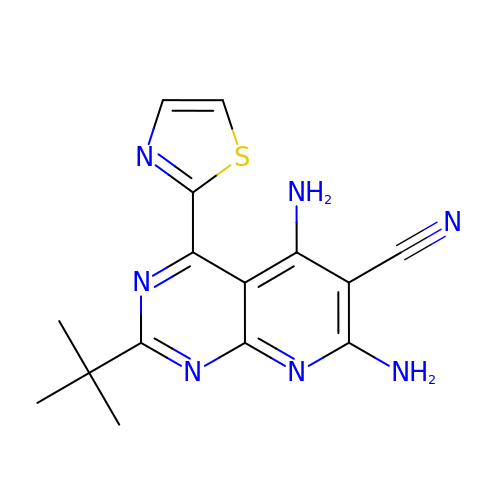5,7-bis(azanyl)-2-tert-butyl-4-(1,3-thiazol-2-yl)pyrido[2,3-d]pyrimidine-6-carbonitrile | C15 H15 N7 S | VDKRFQKJPXSMOG-UHFFFAOYSA-N>[3x]MHTDGDKAFVDFLSDEIKEERKIQKHKTLPKMSGGWELELNGTEAKLVRKVAGEKITVTFNINNSIPPTFDGEEEPSQGQKVEEQEPELTSTPNFVVEVIKNDDGK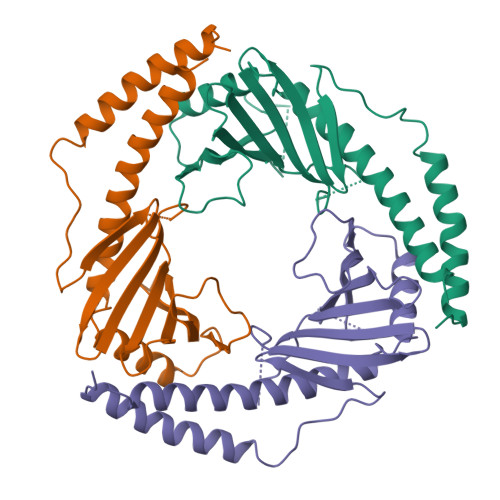KALVLDCHYPEDEVGQEDEAESDIFSIREVSFQSTGESEWKDTNYTLNTDSLDWALYDHLMDFLADRGVDNTFADELVELSTALEHQEYITFLEDLKSFVKSQ> MKHHHHHHHHGGLVPRGSHGGSMENNSLAPLRVGILGFGGLGQAAARLLAPKQEMKLVAVADRHGYLYDADGIDVDNAVQAYTQQGSVGKAKKGQMSEQSIEDLIGEGEVDGYFLALPNLPN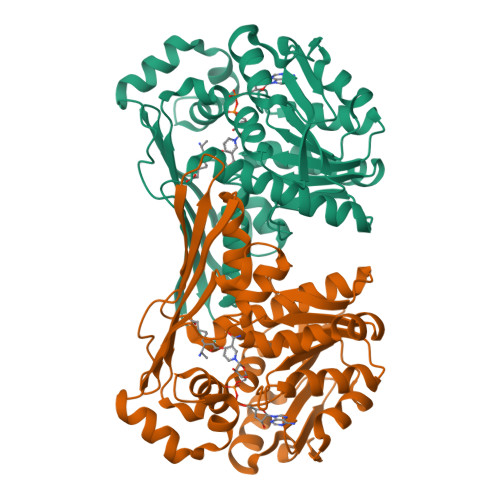TFMADVTRQFIASGWQGVLVDALARTSAVEQLITLREDLAQAGITYMTGCGATPGLLTAAAAIASQSFQEIHQVKITFGVGIANWEAYRATIREDIAHMPGYNVDKAQAMTDAEVAALLDQTNGILALEDMEHADDIMLELAGICHRDQVTVGGVVDTRNPKKPLSTHVKITGRTFEGKISSHTFTLGDETSMAANVCGPAFGYLKAGYGLHRQGLKGLFTAADVMPKFVR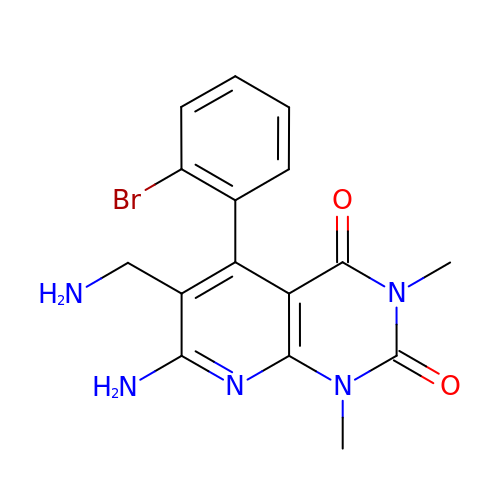7-amino-6-(aminomethyl)-5-(2-bromophenyl)-1,3-dimethylpyrido[2,3-d]pyrimidine-2,4(1H,3H)-dione | C16 H16 Br N5 O2 | JGBNONXELAWFNR-UHFFFAOYSA-N Protein N-glycosylation requires a lipid-linked oligosaccharide (LLO) that acts as a glycan donor of the transfer reaction. Among the various glycosyltransferases (GTs) involved in this process, PglH stands out because it is a membrane-associated enzyme that catalyzes a well-controlled, processive reaction. PglH exhibits the protein fold described for GT-B GTs, consisting of two Rossman-like domains connected by a linker region. To understand the structural basis of such a counting mechanism, we combine structural studies and molecular dynamics simulations with synthetic, chemo-enzymatic, and enzymological studies, and uncover a mechanism by which PglH controls the number of successive glycan transfer reactions using a structural element that not only attaches the protein to the membrane surface, but also contains residues that interact with the pyrophosphate group of the LLO during elongation of the glycan moiety.

The structure of a binary complex with the donor substrate UDP-GalNAc was determined at 2.3 Å resolution, whereas the structures of ternary complexes including synthetic acceptor LLO and either UDP or UDP-CH2-GalNAc were determined at 2.8 Å and 3.3 Å, respectively. The structure of PglH bound to UDP-GalNAc revealed the molecular details of the interactions with the donor substrate. The uridine moiety is positioned in a pocket formed by α12 and the loop connecting α10 and α11. The 2’ and 3’ hydroxyl groups of the ribose moiety form hydrogen bonds with E275, which is part of the conserved EX7E motif along with E267, which interacts with the N-acetyl group of GalNAc. The pyrophosphate moiety interacts via hydrogen bonds with R191, K196, and T271. The GalNAc unit is located in the cleft formed between the N- and C-terminal domains. Unlike in some structural studies of GT-B enzymes, the saccharide moieties were clearly visible not only for the non-hydrolyzable UDP-CH2-GalNAc, but also for the functional UDP-GalNAc. The 6’ hydroxyl of GalNAc forms a hydrogen bond with the side chain of H118. The structure can explain the specificity of PglH for GalNAc over GlcNAc: whereas the axial hydroxyl group at C4 of GalNAc can be accommodated by the enzyme, an equatorial hydroxyl group (present in GlcNAc) would generate a steric clash with the main chain carbonyl oxygen of L269.

>[2x]MMMKISFIIATLNSGGAERVLVTLANALCKEHEVSIIKFHTGESFYKLENEVKVTSLEQFRFDTLYHKIASRFKKFFALRKALKESKADVFISFLDTTNIACILANIGLKTPLIISEHSNEAYLKPKTWRFLRRVSYPFCDALSVLGSSDKVYYERFVKRVKLLLNPCHFSDEIPFDSSFEKENLVLFIGRLDHNKNPVMFLKAIAHLDKNLQENYKFVIAGDGELRQELEYKVKSLGIKVDFLGRVENVKALYEKAKVLCLCSFVEGLPTVLIESLYFEVCRISSSYYNGAKDLIKDNHDGLLVGCDDEIALAKKLELVLNDENFRKELVNNAKQRCKDFEISNIKEEWLKLIVEVKNALGSHHHHHHHHHH> AALPDQSFLWNVFQRVDKDRSGVISDTELQQALSNGTWTPFNPVTVRSIISMFD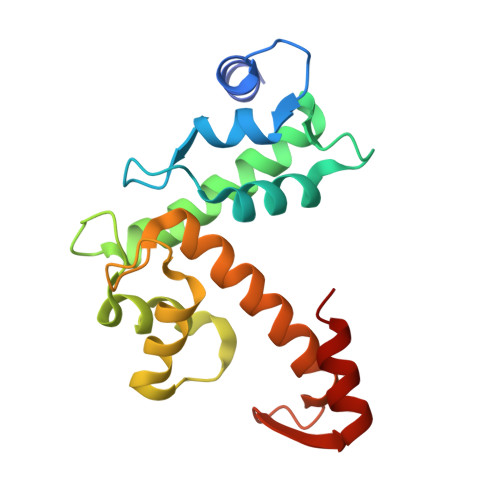RENKAGVNFSEFTGVWKYITDWQNVFRTYDRDNSGMIDKNELKQALSGFGYRLSDQFHDILIRKFDRQGRGQIAFDDFIQGCIVLQRLTDIFRRYDTDQDGWIQVSYEQYLSMVFSIV> GVTFDDGAYTGIREINFEYNSETAIGGLRVTYDLNGMPFVAEDHKSFITGFKPVKISLEFPSEYIVEVS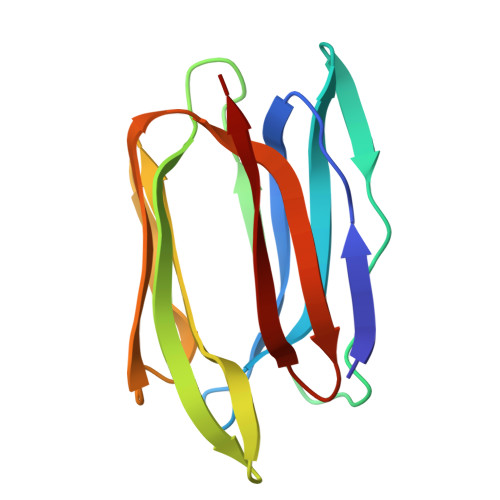GYVGKVEGYTVIRSLTFKTNKQTYGPYGVTNGTPFSLPIENGLIVGFKGSIGYWLDYFSIYLSL> KTYRRSYTHAKPPYSYISLITMAIQQSPNKMLTLSEIYQWIMDLFPFYRQNQQRWQNSIRHSLSFNDCFLKVPRSPDKPGKGSFWTLHPDSGNMFENGCYLRRQKRFKCEKQLALKEAA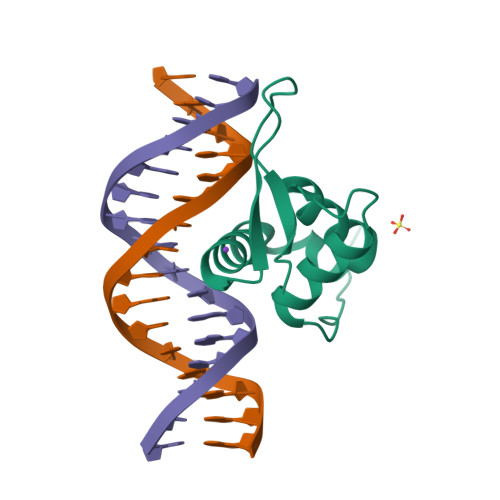GAAGSG>AKDPSWASILQGLEEPYHTFVERLNVALDNGLPEGTPKDPILRSLAYSNANKECQKLLQARGHTNSPLGDMLRACQAWTPKDKTK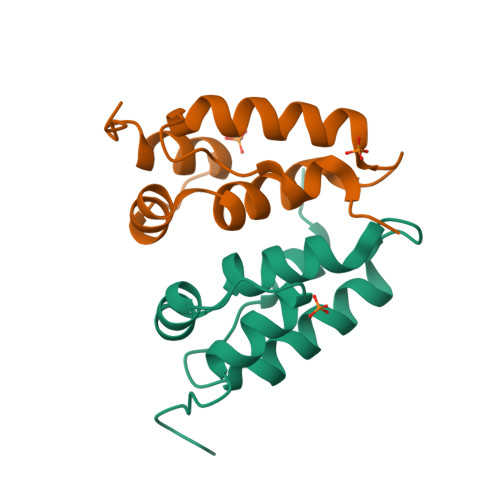VL[6x]>ETGETEPIVLEGKCLVVCDSNPTSDPTGTALGISSAKVAFSAIRSTNHEPSEMSNRTMIIYFDQVLVNIGNNFDSERSTFIAPRKGIYSFNFHVVKVYNRQTIQVSLMLNGWPVISAFAGDQDVTREAASNGVLIQMEKGDRAYLKLERGNLMGGWKYSTFSGF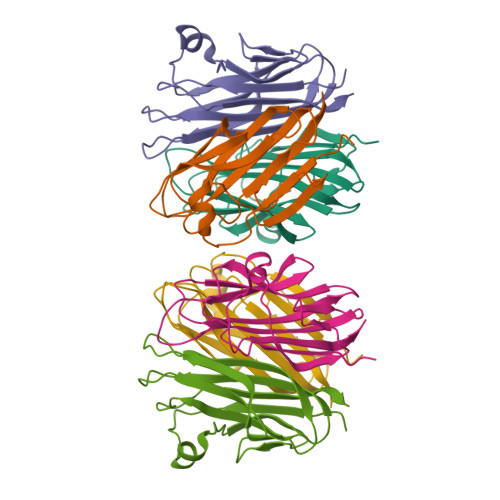LVFPLGTKHHHHHH[4x]>MVRQHAGPRDRSEIVTTSTGTNGRHTVAGPGSAGPVGYSLPLSPTGESAMLTPPPWHFSGEVVMVDYRVDPDAARRFLPPGLEPGADPGAAAAVFATWQWCSQDGAELTDPGRCQFGEFLILLSCEFEGRPMARCPYAWVDQAVPMMRGWVQGMPKQFGVIHQSRPVTVGKAGSRLAPGGRFDGALSVHGRRVVEASVTVDRSTDQPPALHDVPLAHTLVFPEWVPSGGGPRPRLVASEVSDVEFSPIWTGSGDLTFFDGLGD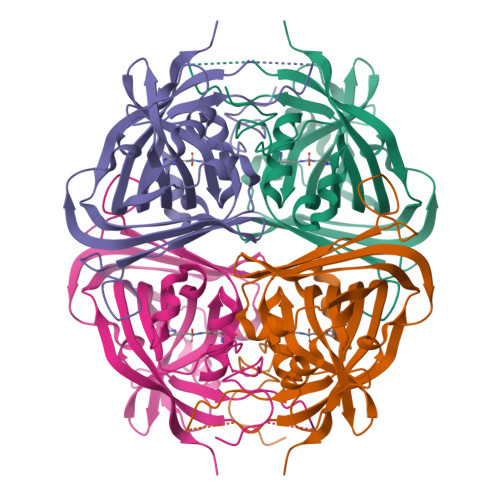DFGALAPLEVGSGHVFSYGETLHGGRLLSDYSVSERHQP[2x]> GEEKKDSKAFIDVSAATLWTAPDSLRPIDVPSATNPVDLWKWTKSMTLDEKLWLTNANKLETQALLGQEVTVVDKKGDWVKVLVHGQPTPRNEEGYPGWMPEKQLTYNQEFADKTNEPFVLVTKPTAILYINPSEKHKSLEVSYNTRLPLLSEDTISYRVLLPNGQKAWLRKNDGTFYRSQNDIPTPAADDLINTGKMFLGLPYIWAGTSG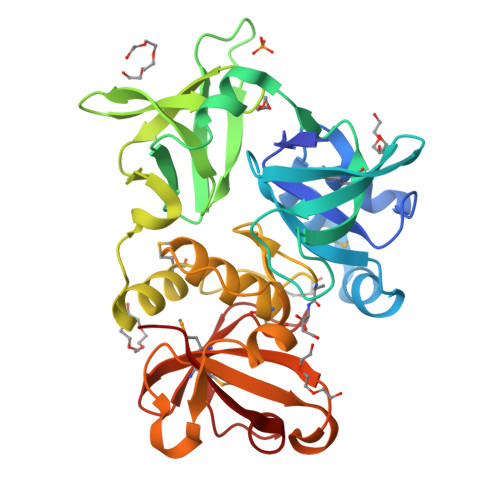FGFDCSGFTHTIYKSHGITIPRDSGPQSRNGVAVDKEHLQKGDLIFFAHDQGKGSVHHVAMYIGDGNMIHSPRAERSVEIIPLNTPGYIEEYAGARRYLP(2R)-3-[(R)-[(1R)-1-amino-3-methylbutyl](hydroxy)phosphoryl]-2-methylpropanoic 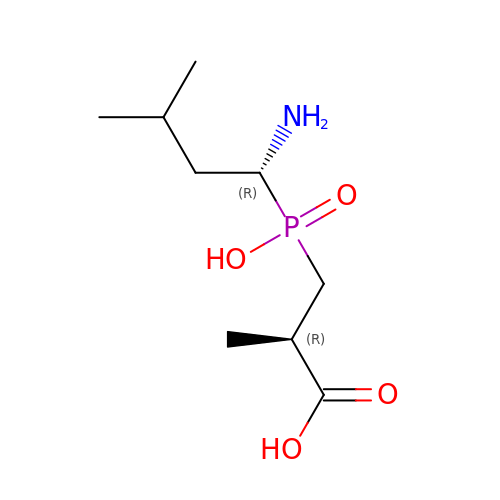acid | C9 H20 N O4 P | PYHFMEIRRPJIRC-JGVFFNPUSA-N> CTAC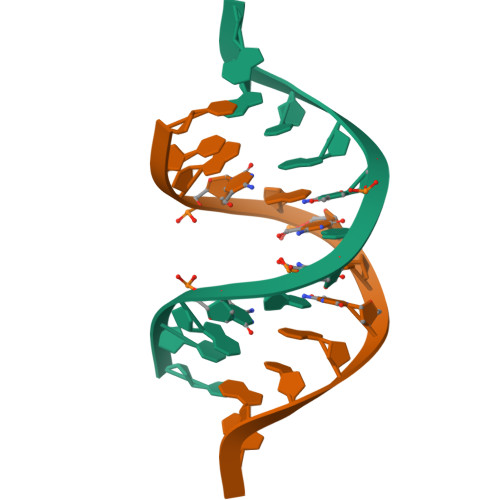GCGCGTAG> GPACPTHADSLNNLANIKREQGNIEEAVRLYRKALE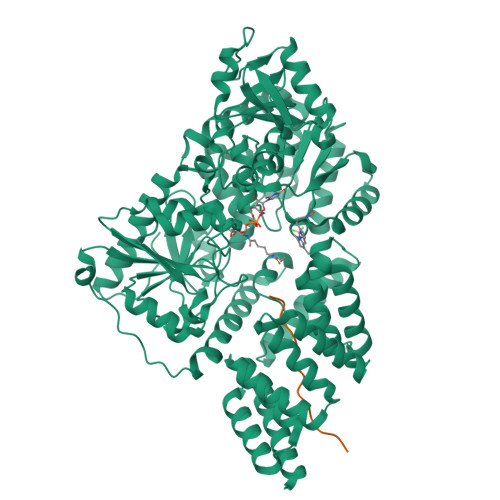VFPEFAAAHSNLASVLQQQGKLQEALMHYKEAIRISPTFADAYSNMGNTLKEMQDVQGALQCYTRAIQINPAFADAHSNLASIHKDSGNIPEAIASYRTALKLKPDFPDAYCNLAHCLQIVCDWTDYDERMKKLVSIVADQLEKNRLPSVHPHHSMLYPLSHGFRKAIAERHGNLCLDKINVLHKPPYEHPKDLKLSDGRLRVGYVSSDFGNHPTSHLMQSIPGMHNPDKFEVFCYALSPDDGTNFRVKVMAEANHFIDLSQIPCNGKAADRIHQDGIHILVNMNGYTKGARNELFALRPAPIQAMWLGYPGTSGALFMDYIITDQETSPAEVAEQYSEKLAYMPHTFFIGDHANMFPHLKKKAVIDFKSNGHIYDNRIVLNGIDLKAFLDSLPDVKIVKMKCPDGGDNADSSNTALNMPVIPMNTIAEAVIEMINRGQIQITINGFSISNGLATTQINNKAATGEEVPRTIIVTTRSQYGLPEDAIVYCNFNQLYKIDPSTLQMWANILKRVPNSVLWLLRFPAVGEPNIQQYAQNMGLPQNRIIFSPVAPKEEHVRRGQLADVCLDTPLCNGHTTGMDVLWAGTPMVTMPGETLASRVAASQLTCLGCLELIAKNRQEYEDIAVKLGTDLEYLKKVRGKVWKQRISSPLFNTKQYTMELERLYLQMWEHYAAGNKPDHMIKPVEVTESA;> THETGTTNTATTATSN>MDVTFLGTGAAYPSPTRGASAVVLRCEGECWLFDCGEGTQTQLMKSQLKAGRITKIFITHLHGDHFFGLPGLLCTISLQSGSMVSKQPIEIYGPVGLRDFIWRTMELSHTELVFHYVVHELVPTADQCPAEELKEFAHVNRADSPPKEEQGRTILLDSEENSYLLFDDEQFVVKAFRLFHRIPSFGFSVVEKKRPGKLNAQKLKDLGVPPGPAYGKLKNGISVVLENGVTISPQDVLKKPIVGRKICILGDCSGVVGDGGVKLCFEADLLIHEATLDDAQMDKAKEHGHSTPQMAAT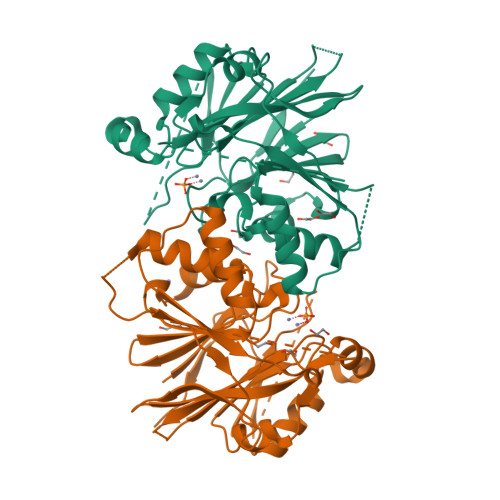FAKLCRAKRLVLTHFSQRYKPVALAREGETDGIAELKKQAESVLDLQEVTLAEDFMVISIPIKKAENLYFQ[2x]>[2x]MATLQDIGVSAGINILSAFVFFIIFAVLRLQPFNDRVYFSKWYLKGLRSSPARGGAFAQRFVNLDFRSYMKFLNWMPEALKMPEPELIDHAGLDSVVYLRIYWLGLKIFTPIAVLAWAVLVPVNWTNNTLEMAKQLRNVTSSDIDKLSVSNIPEYSMRFWTHIVMAYAFTIWTCYVLMKEYETIANMRLQFVASEARRPDQFTVLVRNVPPDADESVSELVEHFFLVNHPDHYLTHQVVCNANKLADLVKKKKKLQNWLDYYQLKYARNNSQRIMVKLGFLGLWGQKVDAIEHYIAEIDKISKEISKEREEVVNDPKAIMPAAFVSFKTRWAAAVCAQTQQTRNPTQWLTEWAPEPRDVFWSNLAIPYVSLTVRRLIMHVAFFFL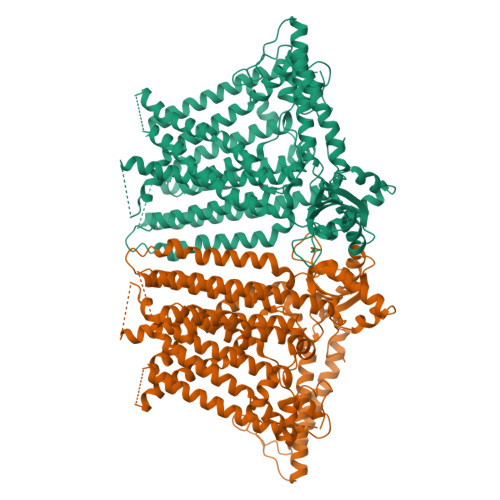TFFFIVPIAFVQSLATIEGIVKAAPFLKFIVDDKFMKSVIQGFLPGIALKLFLAFLPSILMIMSKFEGFTSISSLERRAAFRYYIFNLVNVFLASVIAGAAFEQLNSFLNQSANQIPKTIGVAIPMKATFFITYIMVDGWAGVAGEILMLKPLIMFHLKNAFLVKTDKDREEAMDPGSIGFNTGEPRIQLYFLLGLVYAPVTPMLLPFILVFFALAYIVYRHQIINVYNQEYESAAAFWPDVHGRVIAALVISQLLLMGLLGTKHAALAAPFLIALPVLTIGFHHFCKGRYEPAFIRYPLQEAMMKDTLETAREPNLNLKGYLQNAYVHPVFKGDEDDYDIDDKLGKFEDEAIIVPTKRQSRRNTPAPSIISGDDSPSLPFSGKLVGTGTLEVLFQ>[4x]SGSGKPSYQIYMEIFETKQSYDEVIDSFICKQRALL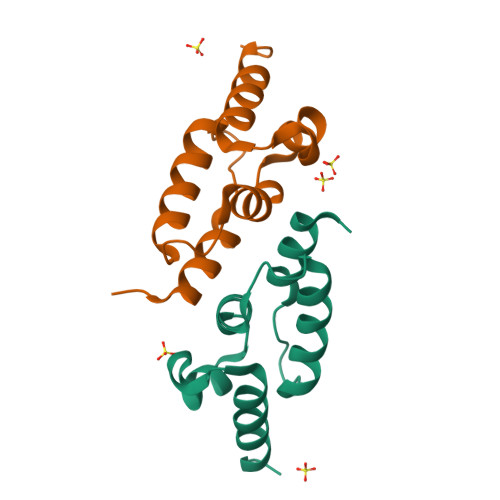AKLPEGRHDEETELDFIYGLMQPKYRESIPRHEVKTFRELLDRGRTVERTRH> TTHFTVADRWGNVVSYTTTIEQLFGTGIMVPDYGVILNNELTDFDAIPGGANEVQPNKRPLSSMT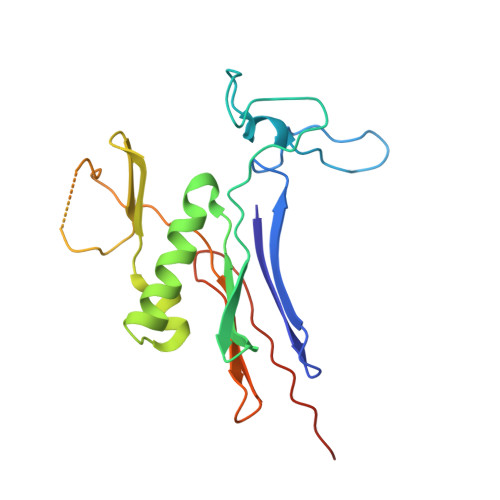PTILFKDDKPVLTVGSPGGATIISSVLQTILYHIEYGMELKAAVEEPRIYTNSMSSYRYEDGVPKDVLSKLNGMGHKFGTSPVDIGNVQSISIDHENGTFKGVADSSRNGAAIGINLKRKLEHHHHHH>[5x]MAMTLRDMDAVRPVNREAVDRHKARMRDEVRAFRLRELRAAQSLTQVQVAALAHIR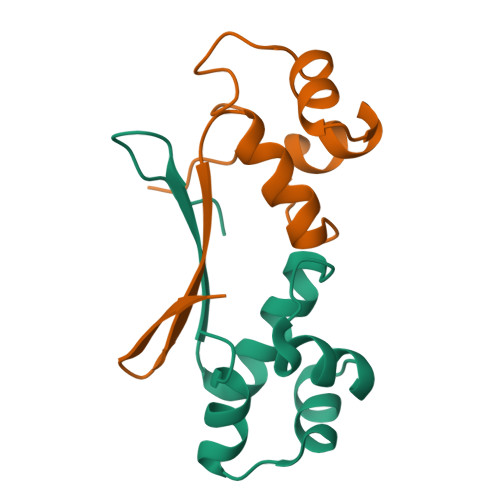QSRVSSIENGDIGSAQVNTLRKYVSALGGELDITVRLGDETFTLA> MDIVKLRELLEAELSSTDLNELDEDFYVEFDSLIKALKLSAESSRERGEDVEERLYLAQLKIAESLMKEIIKLRLHKIVDLAVEGKIAEMTAEEKRLFNVIRAFIEREELPEISEEVQPQEESEAEAEYRSKEVPKEAY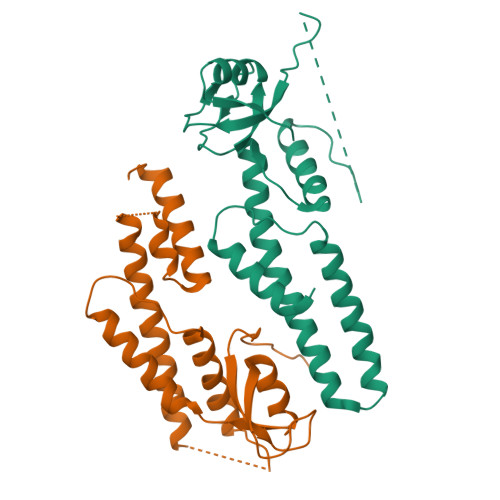IIQIDLPAVLGPDMKEYGPFMAGDMAIIPTVIGRALVEREAARRVRIFL;> NYFQGSHMFTGKALIAVKVMKPFGDWKSGDIVLVEDWKARELWEAGVVEIVDETDKIIGEIDKVIAEERESEPLTLLPEGLYERAEFYAYYLENYVRLNPRESVDTINVKLTKLANLRKKLRDLKLIRFNKILKAVMLRPNSLELLSRLAPEERRIYLQMSKIRNEWLGDA> ADKELKFLVVDKFSTMRRIVRNLLKELGFNNVEEAEDGVDALNKLQAGGYGFVISDWNMPNMDGLELLKTIRADGAMSALPVLMVTAEAK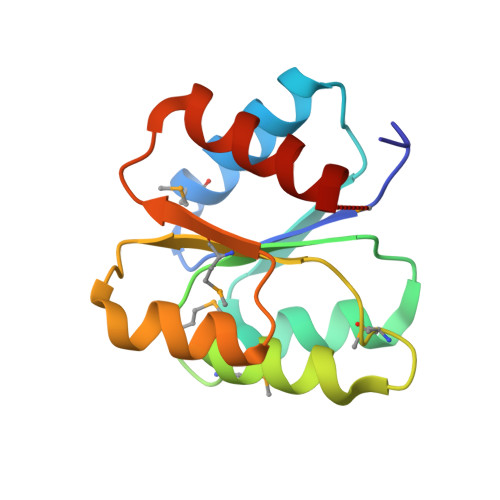KENIIAAAQAGASGWVVKPFTAATLEEKLNKIFEKLGM> QEDFPPRIVEHPSDLIVSK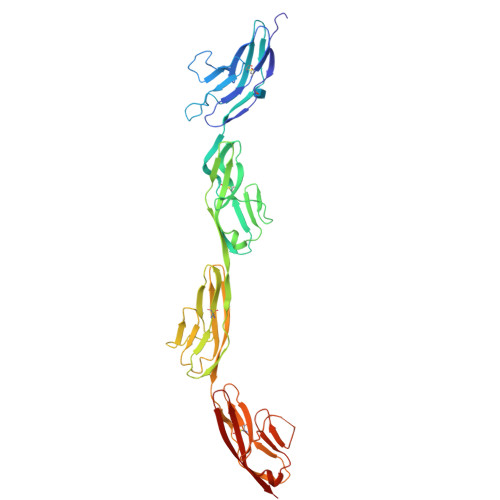GEPATLNCKAEGRPTPTIEWYKGGERVETDKDDPRSHRMLLPSGSLFFLRIVHGRKSRPDEGVYVCVARNYLGEAVSHNASLEVAILRDDFRQNPSDVMVAVGEPAVMECQPPRGHPEPTISWKKDGSPLDDKDERITIRGGKLMITYTRKSDAGKYVCVGTNMVGERESEVAELTVLERPSFVKRPSNLAVTVDDSAEFKCEARGDPVPTVRWRKDDGELPKSRYEIRDDHTLKIRKVTAGDMGSYTCVAENMVGKAEASATLTVQEPPHFVVKPRDQVVALGRTVTFQCEATGNPQPAIFWRREGSQNLLFSYQPPQSSSRFSVSQTGDLTITNVQRSDVGYYICQTLNVAGSIITKAYLEVTG>[2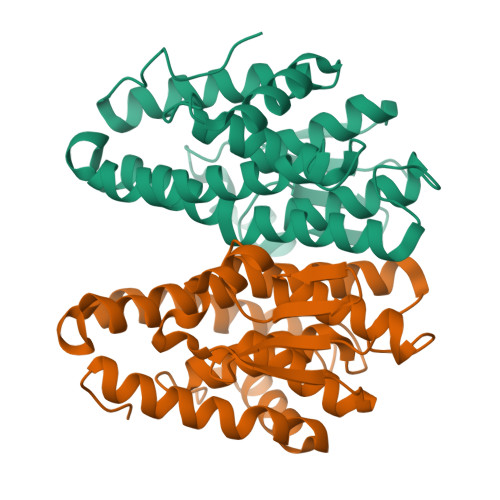x]MNHKVHMMSQPKPILYYDERSPPVRSCLMLIKLLDIDVELRFVNLFKGEQFQKDFLALNPQHSVPTLVHGDLVLTDSHAILIHLAEKFDEGGSLWPQEHAERMKVLNLLLFECSFLFRRASDFMSAIVRQGFANVDVAHHERKLTEAYIIMERYLENSDFMAGPQLTLADLSIVTTLSTVNLMFPLSQFPRLRRWFTAMQQLDAYEANCSGLEKLRQTMESVGSFQFPSSSAVVTEKVE> MNSEQLLHNYVSDSLLTTLISFQEFKQQLQSYTSDEQQLQHWYELLQARDARVTS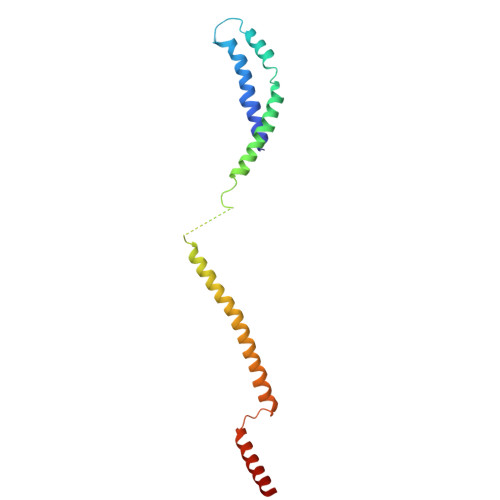ELEARIKQFFITLRSRLLRFLESEQLSHSLSLETLIDALYKINDLLQQRLQILDDAIQEKTSELAEFENMVRSPSAGDNAIPGLLQIIQSYINLLEEN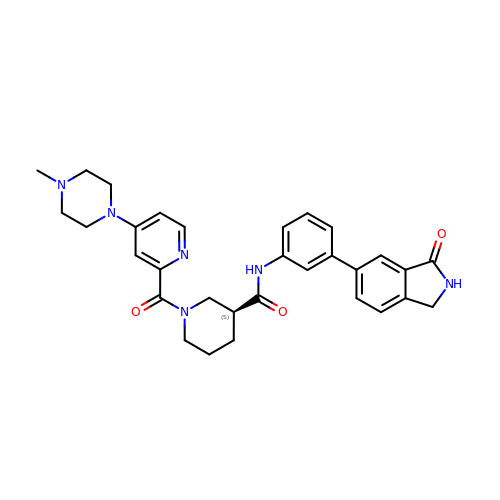(3S)-1-[4-(4-methylpiperazin-1-yl)pyridine-2-carbonyl]-N-[(3M)-3-(3-oxo-2,3-dihydro-1H-isoindol-5-yl)phenyl]piperidine-3-carboxamide | C31 H34 N6 O3 | OYWGFOXQBJYTIR-DEOSSOPVSA-N> YEMSSVGVINLRNMYSTYDPTEVKGKINEGPPFSGSLFYKNIPYGNSSIELKVEMNSVEKANFFSGKRVDIFTLEYSPPSNSNIKKNSYGGITLSDGNRIDKKNIPVNIFIDGVQQKYSYTDISTVSTDKKEVTIQELDVKSR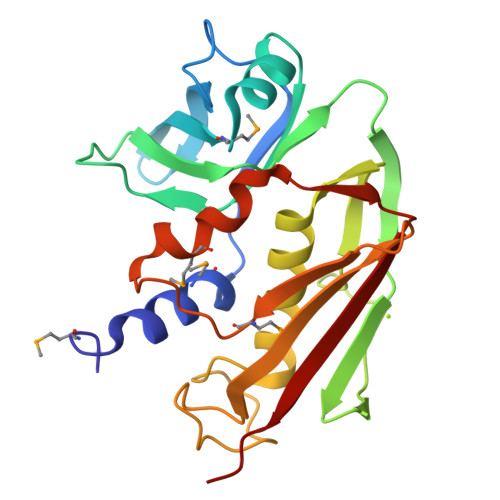YYLQKHFNIYGFGDVKDFGRSSRFQSGFEEGNIIFHLNSGERISYNMFDTGHGDRESMLKKYSDNKTAYSDQLHIDIYLVKFNK>[8x]MSYYHHHHHHLESTSLYKKAGFENLYFQGSGAMSVLQYTEISNISSDKINI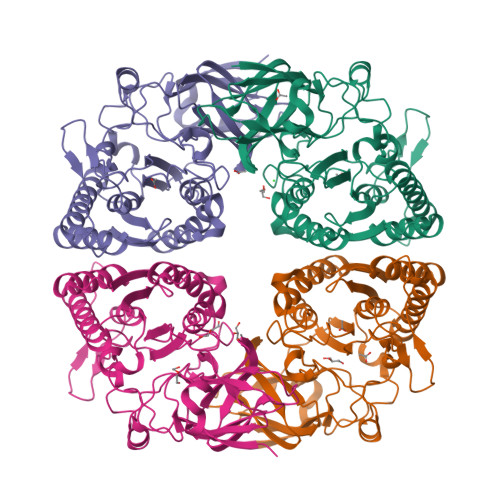LGRTGKKRQPLPVFFNGGGVEVVVTGSELWIDLETDSDVNEMWVALEINGAFIARQMLLPGEHSLCLFRSMEKTTPKRVRLYRELQAMNDDPKVKLLFKGFKHDGEFQNVPVYSRKLEFIGDSITSGEGSYGAFDDVDWIPMYMSASANYATMTAKALNADYHLVSQGGWGVFCGWDNDVRHNLPSVYEKVCGLAKGEMNEELGAQEEYDFASWQPDAIIVNLGTNDVTSFNQPEFLNPDDGKTYKMRTNTDGTRNREDELKIVSAIIDFLTMLRKHNPNAQIIWSYGMLGSDLNLVITEGINKYKENAGDEKVSFFQLPNTTMENFGSHMAPGPKSHQNAAKELVDYLRNKLGWFE> GSHMSEWKARRFWASVGIHKEEGGWAVLLDERPLRTPGKQPLRLPTEALALAIAEEWQAVQEVIDPNAMPLTRSANSAIEKVAPQFDAVAAMLGDYGGTDLLSYRADAPEALVRAQAEGWDPL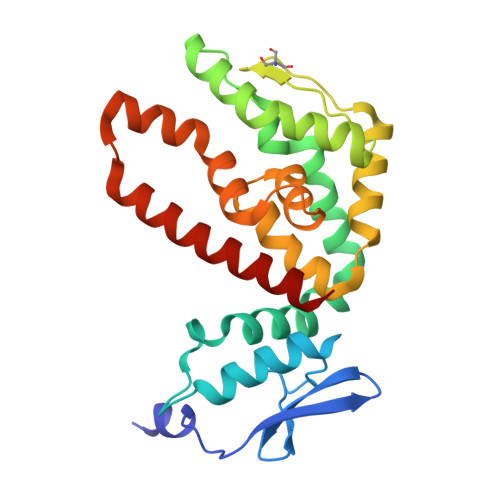IDWAATELRAPLRITHGVIPVPQDPVVLLKLRAEVASLDPFGLTALHDLVTLPGSLILGLAVIRGRIDAPTAHALSRIDEEFQAERWGRDEEAEAQAASRLAAMRDSERFWHLTRG> GPHMSYDASAIRVLKGLEGVRHRPAMYIGGTGVEGYHHLFKEILDNAVDEALAGYATEILVRLNEDGSLTVEDNGRGIPVDLMPEEGKPAVEVIYTTLHSGGKFEQGAYKVSGGLHGVGASVVNALSEWTVVEVFREGKHHRIAFSRGEVTEPLRVVGEAPRGKTGTRVTFKPDPEIFGNLRFDPSKIRARLREVAYLVAGLKLVFQDRQHGKEEVFLDKGGVASFAKALAEGEDLLYEKPFLIRGTHGEVEVEVGFLHTQGYNAEILTYANMIPTRDGGTHLTAFKSAYSRALNQYAKKAGLNKEKGPQPTGDDLLEGLYAVVSVKLPNPQFEGQTKGKLLNPEAGTAVGQVVYERLLEILEENPRIAKAVYEKALRAAQ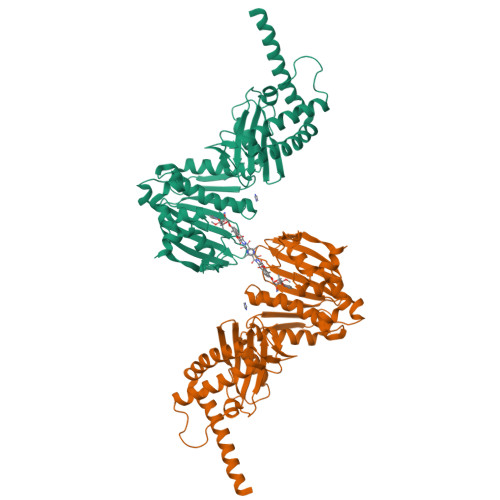AREAARKARELV> GHMLQNNTDYPFEANNPYMYHENPMEEGLSMLKLANLAEAALAFEAVCQAAPEREEAWRSLGLTQAENEKDGLAIIALNHARMLDPKDIAVHAALAVSHTNEHNANAALASLRAWLLSQPQYEQLGSVNLQADVDIDDLNVQSEDFFFAAPNEYRECRTLLHAALEMNPNDAQLHASLGVLYNLSNNYDSAAANLRRAVELRPDDAQLWNKLGATLANGNRPQEALDAYNRALDINPGYVRVMYNMAVSYSNMSQYDLAAKQLVRAIYMQVGGTTPTGEASREAT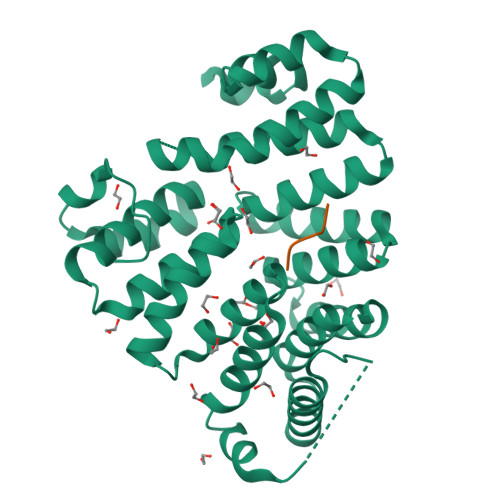RSMWDFFRMLLNVMNRPDLVELTYAQNVEPFAKEFGLQSMLL;> RDRAAKL> RKAENKYAGGNP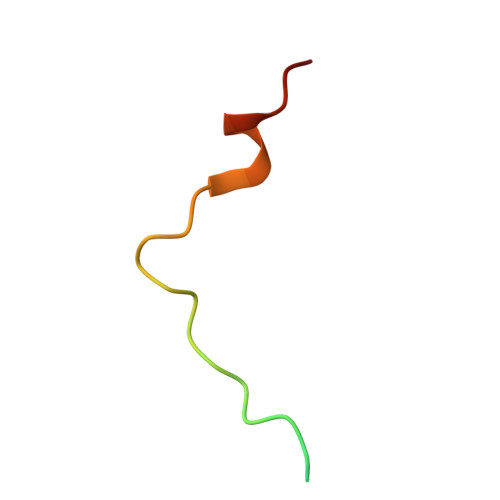VCVRPTPKWQKGIGEFFRLS>DEPVTYEEEAVPAPVRGRLEVLSDLLYVASPDRAMVFTRTKAETEEIAQGLLRLGHPAQALHGDLSQGERERVLGAFRQGEVRVLVATDVAARGLDIPQVDLVVHYRLPDRAEAYQHRSGRTGRAGRGGRVV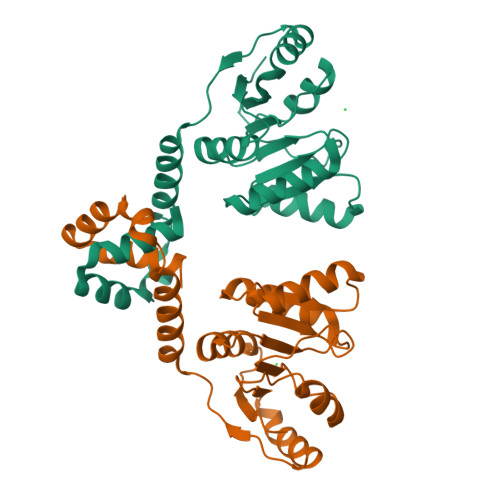LLYGPRERRDVEALERAVGRRFKRVNPPTPEEVLEAKWRHLLARLARVPEKDYRLYQDFAGRLFAEGRVEVVAALLALLL[2x]> MVGGGTVKKDL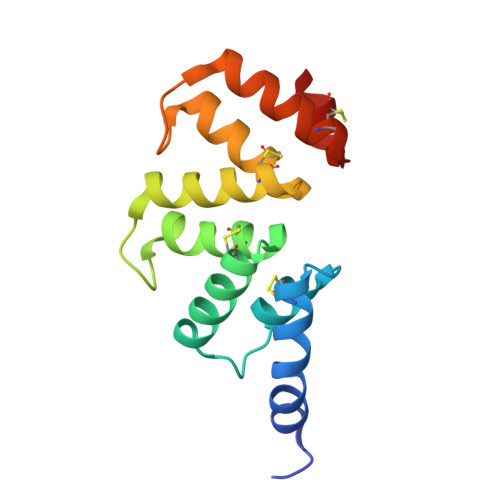KKAIQYYVKACELNEMFGCLSLVSNSQINKQKLFQYLSKACELNSGNGCRFLGDFYENGKYVKKDLRKAAQYYSKACGLNDQDGCLILGYKQYAGKGVVKNEKQAVKTFEKACRLGSEDACGILNNY> MHHHHHHSSGRENLYFQGTFAERYNIVCMLGKGSFGEVLKCKDRITQQEYAVKVINKASAKNKDTSTILREVELLKKLDHPNIMKLFEILEDSSSFYIVGELYTGGELFDEIIKRKRFSEHDAARIIKQVFSGITYMHKHNIVHRDLKPENILLESKEKDCDIKIIDFGLSTCFQQNTKMKDRIGTAYYIAPEVLRGTYDEKCDVWSAGVILYILLSGTP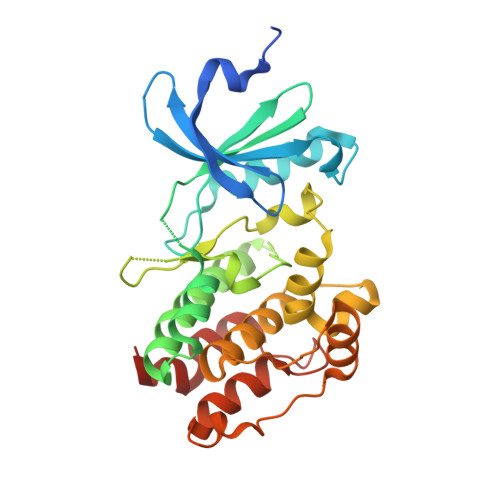PFYGKNEYDILKRVETGKYAFDLPQWRTISDDAKDLIRKMLTFHPSLRITATQCLEHPWIQKYSSE>MDRASELLFYVNGRKVIEKNVDPETMLLPYLRKKLRLTGTKYGCGGGGCGACTVMISRYNPITKRIRHHPANACLIPICSLYGAAVTTVEGIGSTHTRIHPVQERIAKCHGTQCGFCTPGMVMSIYTLLRNHPEPTLDQLTDALGGNLCRCTGYRPIIDACKTFCKTSGCCQSKENGVCCLDQGINGLPEFEEGSKTSPKLFAEEEFLPLDPTQELIFPPELMIMAEKQSQRTRVFGSERMMWFSPVTLKELLEFKFKYPQAPVIMGNTSVGPEVKFKGVFHPVIISPDRIEELSVVNHAYNGLTLGAGLSLAQVKDILADVVQKLPEEKTQMYHALLKHLGTLAGSQIRNMASLGGHIISRHPDSDLNPILAVGNCTLNLLSKEGKRQIPLNEQFLSKCPNADLKPQEILVSVNIPYSRKWEFVSAFRQAQRQENALAIVNSGMRVFFGEGDGIIRELCISYGGVGPATICAKNSCQKLIGRHWNEQMLDIACRLILNEVSLLGSAPGGKVEFKRTLIISFLFKFYLEVSQILKKMDPVHYPSLADKYESALEDLHSKHHCSTLKYQNIGPKQHPEDPIGHPIMHLSGVKHATGEAIYCDDMPLVDQELFLTFVTSSRAHAKIVSIDLSEALSMPGVVDIMTAEHLSDVNSFCFFTEAEKFLATDKVFCVGQLVCAVLADSEVQAKRAAKRVKIVYQDLEPLILTIEESIQHNSSFKPERKLEYGNVDEAFKVVDQILEGEIHMGGQEHFYMETQSMLVVPKGEDQEMDVYVSTQFPKYIQDIVASTLKLPANKVMCHVRRVGGAFGGKVLKTGIIAAVTAFAANKHGRAVRCVLERGEDMLITGGRHPYLGKYKAGFMNDGRILALDMEHYSNAGASLDESLFVIEMGLLKMDNAYKFPNLRCRGWACRTNLPSNTAFRGFGFPQAALITESCITEVAAKCGLSPEKVRIINMYKEIDQTPYKQEINAKNLIQCWRECMAMSSYSLRKVAVEKFNAENYWKKKGLAMVPLKFPVGLGSRAAGQAAALVHIYLDGSVLVTHGGIEMGQGVHTKMIQVVSRELRMPMSNVHLRGTSTETVPNANISGGSVVADLNGLAVKDACQTLLKRLEPIISKNPKGTWKDWAQTAFDESINLSAVGYFRGYESDMNWEKGEGQPFEYFVYGAACSEVEIDCLTGDHKNIRTDIVMDVGCSINPAIDIGQIEGAFIQGMGLYTIEELNYSPQGILHTHGPDQYKIPAICDMPTELHIALLPPSQNSNTLYSSKGLGESGVFLGCSVFFAIHDAVSAARQ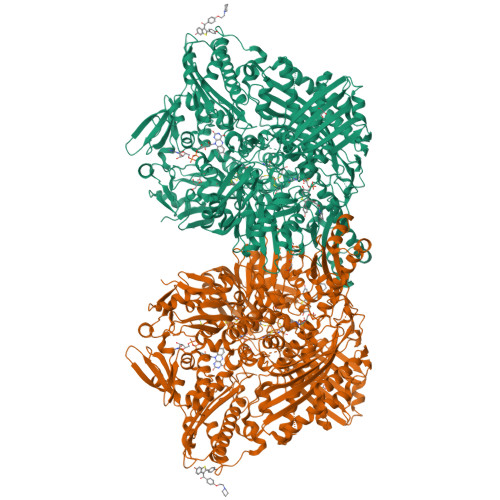ERGLHGPLTLNSPLTPEKIRMACEDKFTKMIPRDEPGSYVPWNVPI[2x]> MLNQFPGQYSNNI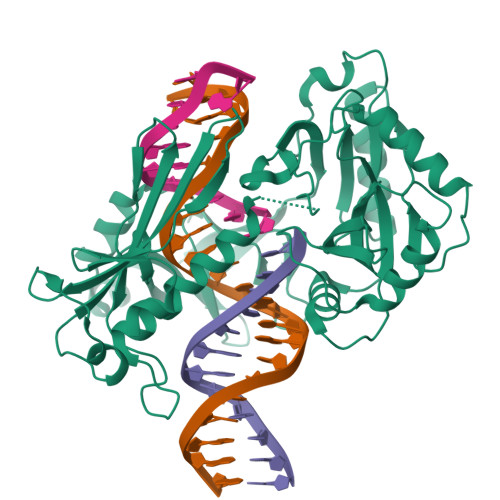FCFPPIESETKSGKKASWIICVQVVQHNTIIPITDEMFSTDVKDAVAEIFTKFFVEEGAVRISKMTRVTEGKNLGKKNATTVVHQAFKDALSKYNRHARQKRGAHTNRGMIPPMLVKYFNIIPKTFFEEETDPIVQRKRNGVRAVACQQGDGCILLYSRTEKEFLGLDNIKKELKQLYLFIDVRVYLDGELYLHRKPLQWIAGQANAKTDSSELHFYVFDCFWSDQLQMPSNKRQQLLTNIFKQKEDLTFIHQVENFSVKNVDEALRLKAQFIKEGYEGAIVRNANGPYEPGYNNYHSAHLAKLKPLLDAEFILVDYTQGKKGKDLGAILWVCELPNKKRFVVTPKHLTYADRYALFQKLTPALFKKHLYGKELTVEYAELSPKTGIPLQARAVGFREPINVLEII>MSGTLYIVSAPSGAGKTSLVKALLDAAPEVRVSVSHTTRGMRPGEVDGVNYHFTSREEFLAMLERNEFLEHAEVFGNLYGTSQRWVEKTLAEGLDLILEIDWQGAQQVRRLMPEAQSIFILPPSQEALRQRLTNRGQDSDEVIERRMREAVSEMSHYVEYDHLVI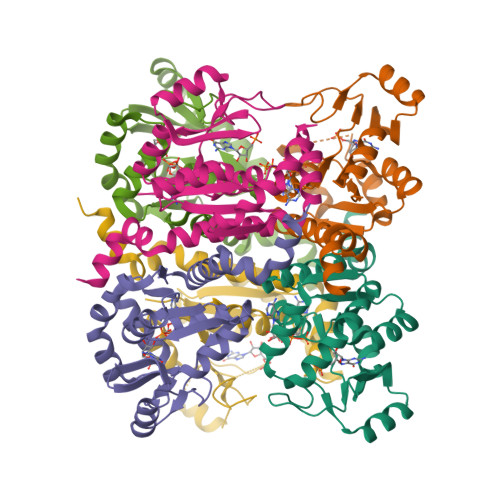NDDFAHALDDLKAIFRARQLRQDAQQQRHAELLGRLLAGHHHHHH[12x]>MSEGPKKAGVLGSPIAHSRSPQLHLAAYRALGLHDWTYERIECGAAELPVVVGGFGPEWVGVSVTMPGKFAALRFADERTARADLVGSANTLVRTPHGWRADNTDIDGVAGALGAAAGHALVLGSGGTAPAAVVGLAELGVTDITVVARNSDKAARLVDLGTRVGVATRFCAFDSGGLADAVAAAEVLVSTIPAEVAAGYAGTLAAIPVLLDAIYDPWPTPLAA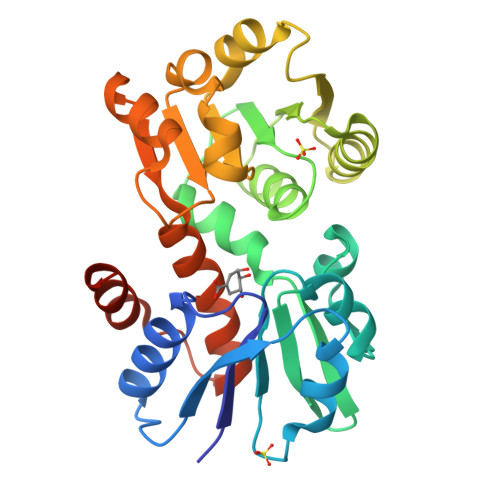AVGSAGGRVISGLQMLLHQAFAQVEQFTGLPAPREAMTCALAALDLDHHHHHH[3x]>MSLKITKIEIFHVHTRPQSGQRPILVKVSTDEGIYGLGEAGIAYGVGGSAAAGILKDYAALLIGEDPFNTEAIWEKLFKKTFWGQGGGTVIFSGISAFDIAFWDIKGKALNLPVYKLLGGKNREDLRVYASQLQFGWGKERKSKGRKEEYAEEALKAVAEGYDAVKVDVLAHDRNGSREGVFLEGPLPSETIKIGVERVEAIRNAVGPDVDIIVENHGHTDLVSAIQFAKAIEEFNIFFYEEINTPLNPRLLKEAKKKIDIPLASGERIYSRWGFLPFLEDRSIDVIQPDLGTCGGFTEFKKIADMAHIFEVTVQAHVAGTGVAEAASLHAEIAIPNFCIHEHHQKTLLPEYEELCVHN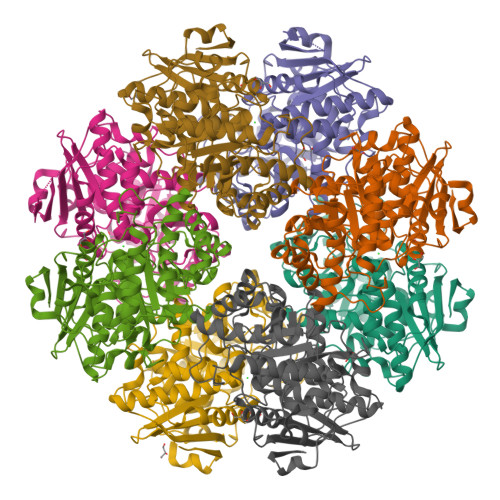YQPVKGRYKVPELPGIGQDITEKLYQISDYVSIEASEGHHHHHH[8x]5'-O-[(4-cyano-2-hydroxybenzoyl)sulfamoyl]adenosine | C18 H17 N7 O8 S | 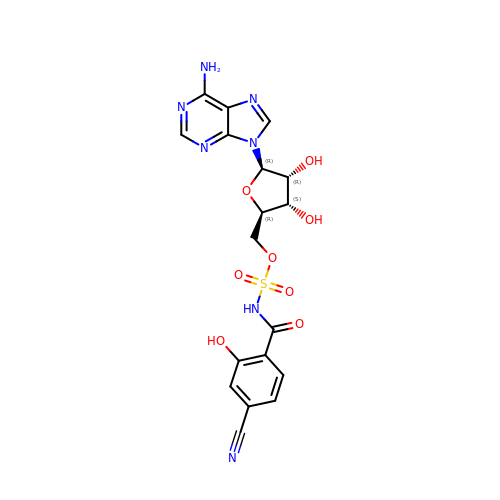WCJMOPOQHFMEGK-XWXWGSFUSA-N> MAYPDANLLNDRVLRAMLKAEETCAPSVSYFKCVQKEVLPSMRKIVATWMLEVCEEQKCEEEVFPLAMNYLDRFLSLEPVKKSRLQLLGATCMFVASKMKETIPLTAEKLCIYTDN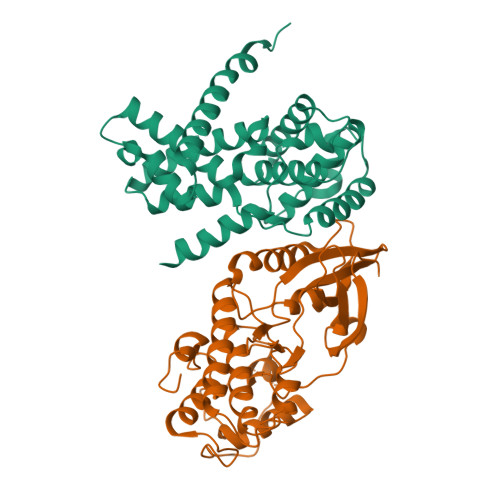SIRPEELLQMELLLVNKLKWNLAAMTPHDFIEHFLSKMPEAEENKQIIRKHAQTFVALCATDVKFISNPPSMVAAGSVVAAVQGLNLRSPNNFLSYYRLTRFLSRVIKCDPDCLRACQEQIEALLESSLRQAQQNMDPKAA;> MATSRYEPVAEIGVGAYGTVYKARDPHSGHFVALKSVRVPNGEEGLPISTVREVALLRRLEAFEHPNVVRLMDVCATSRTDREIKVTLVFEHVDQDLRTYLDKAPPPGLPAETIKDLMRQFLRGLDFLHANCIVHRDLKPENILVTSGGTVKLADFGLARIYSYQMALAPVVVTLWYRAPEVLLQSTYATPVDMWSVGCIFAEMFRRKPLFCGNSEADQLGKIFDLIGLPPEDDWPRDVSLPRGAFPPRGPRPVQSVVPEMEESGAQLLLEMLTFNPHKRISAFRALQHSYLHKDEGNPEHHHHHH> GGIVNVSERHSCPLGFGHYSVVDVCIFETVVIVLLTFLIIAGNLTVIFVFHCAPLLHHYTTSYFIQTMAYADLFVGVSCLVPTLSLLHYSTGVHESLTCQVFGYIISVLKSVSMWCLACISVDRYLAITKPLSYNQLVTPCRLRICIILIWIYSCLIFLPSFFGWGKPGYHGDIFEWCATSWLTSAYFTGFIVCLLYAPAAFVVCFTYFHIFKICRQHTKMKKYTCTVCGYIYNPEDGDPDNGVNPGTDFKDIPDDWVCPLCGVGKDQFEEVEEYLMVLFRIT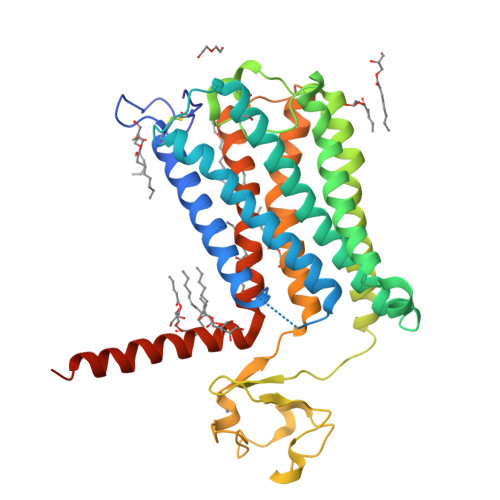SVFYMLQLPYIIYFLLESSRVLDNPTLSFLTTWLAISNSFCNPVIYALSDSTFRLGLRRLSETMCTSCMEFLEVLFQGPHHHHHHHHHH> MSSTMKDTQEAPVRWSRNWTPDAIRALVDQDNGKLDARIYADQDLYQLELERVFGRSWLMLGHETHIPKIGDYLTTYMGEDPVIMVRQKDQSIKVFLNQCRHRGMRIVRSDGGNAKAFTCTYHGWAYDIAGNLVNVPFEKEAFCDKKEGDCGFDKADWGPLQARVETYKGLVFANWDPEAPDLKTYLSDA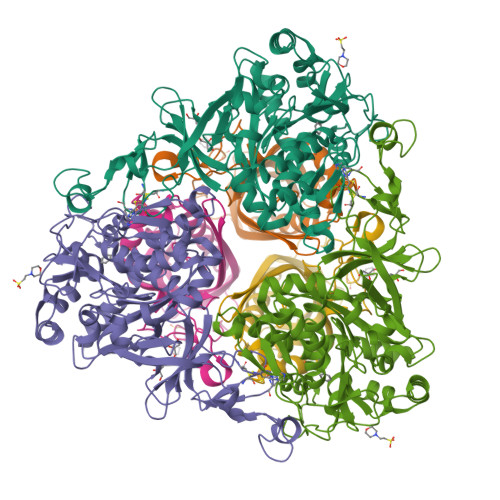MPYMDVMLDRTEAGTEAIGGIQKWVIPCNWKFAAEQFCSDMYHAGTMSHLSGVLAGLPPEMDLTQIQLSKNGNQFRSAWGGHGAGWFINDSSILLSVVGPKITQYWTQGPAAEKAARRVPQLPILDMFGQHMTVFPTCSFLPGINTIRTWHPRGPNEVEVWAFVLVDADAPEDIKEEFRLQNIRTFNAGGVFEQDDGENWVEIQRVMRGHKAKSTSLCAKMGLNVPNKNNPAYPGKTAYVYAEEAARGMYHHWSRMMSEPSWDTLKP;> MISTPLSKEFEWPAKPVSLELQHQVEQFYYREAQLLDHHAFQAWFALLAEDIHYWMPIRTVRTAREQGLEYVPAGANAHFDDTHATMYGRIRQKTSDLNWAEDPPSRTRHLVSNVIVREMDTPGTLEVASAFLLYRSRLERQVDVFAGERRDVLRIADNPLGFQIAKRTIILDQSTVLANNLSVFF> MKKIIYIATIGITLLTTSCDDFLDRQVPQGIVTGDQIASPEYVDNLVISAYAIWATGDDINSSFSLWNYDVRSDDCYKGGSGTEDGGVFNALEISKGINTTDWNINDIWKRLYQCITRANTALQSLDQMDEKTYPLKNQRIAEM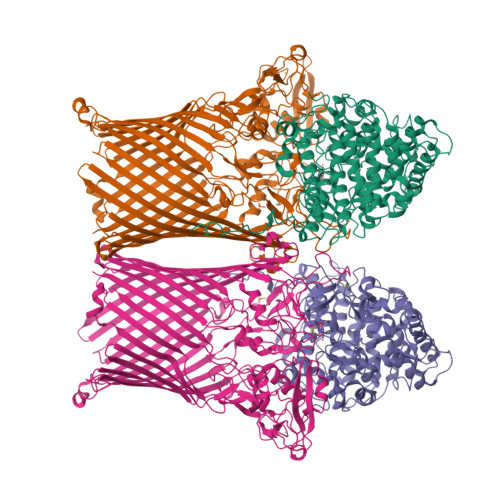RFLRGHAHFMLKQLFKKIVIVNDENMEPDAYNELSNTTYTNDEQWQKIADDFQFAYDNLPEVQIEKGRPAQAAAAAYLAKTYLYKAYRQDGADNALTGINEEDLKQVVKYTDPLIMAKGGYGLETDYSMNFLPQYENGAESVWAIQYSINDGTYNGNLNWGMGLTTPQILGCCDFHKPSQNLVNAFKTDSQGKPLFSTYDNENYEVATDNVDPRLFHTVGMPGFPYKYNEGYIIQKNDDWSRSKGLYGYYVSLKENVDPDCDCLKKGSYWASSLNHIVIRYADVLLMRAEALIQLNDGRITDAISLINEVRSRAAGSTMLIFNYKEDYGVNFKVTPYDLKAYAQDEAMKMLKWERRVEFGMESSRFFDLVRWGEAKDVINAYYVTEASRCSIYKNAGFTENKNEYLPVPFEQISASNGNYTQNFGWAAAAHHHHHH;> MPGIMKNKKLLCSVCFLFAFMSALWGQNITVKGNVTSKTDGQPIIGASVVETTATTNGTITDFDGNFTLSVPVNSTLKITYIGYKPVTVKAAAIVNVLLEEDTQMVDEVVVTGYTTQRKADLTGAVSVVKVDEIQKQGENNPVKALQGRVPGMNITADGNPSGSATVRIRGIGTLNNNDPLYIIDGVPTKAGMHELNGNDIESIQVLKDAASASIYGSRAANGVIIITTKQGKKGQIKINFDASVSASMYQSKMNVLNTEQYGRAMWQAYVNDGENPNGNALGYAYNWGYNADGNPVLYGMTLSKYLDSKNTMPVADTDWFDEITRTGVIQQYNLSVSNGSEKGSSFFSLGYYKNLGVIKDTDFDRFSARMNSDYKLIDDILTIGQHFTLNRTSEVQAPGGIIETALDIPSAIPVYASDGSWGGPVGGWPDRRNPRAVLEYNKDNRYTYWRMFGDAYVNLTPFKGFNLRSTFGLDYANKQARYFTYPYQEGTQTNNGKSAVEAKQEHWTKWMWNAIATYQLEVGKHRGDVMIGMELNREDDSHFSGYKEDFSILTPDYMWPDAGSGTAQAYGAGEGYSLVSFFGKMNYSYADRYLLSLTLRRDGSSRFGKNHRYATFPSVSLGWRITQENFMKELTWLDDLKLRASWGQTGNQEISNLARYTIYAPNYGTTDSFGGQSYGTAYDITGSNGGGVLPSGFKRNQIGNDNIKWETTTQTNVGIDFSLFKQSLYGSLEYYYKKATDILTEMAGVGVLGEGGSRWINSGAMKNQGFEFNLGYRNKTAFGLTYDLNGNISTYRNEILELPETVAANGKFGGNGVKSVVGHTYGAQVGYIADGIFKSQDEVDNHATQEGAAVGRIRYRDIDHNGVIDERDQNWIYDPTPSFSYGLNIYLEYKNFDLTMFWQGVQGVDIISDVKKKSDFWSASNVGFLNKGTRLLNAWSPTNPNSDIPALTRSDTNNEQRVSTYFVENGSFLKLRNIQLGYTVPAVISKKMRMDRLRFYCSAQNLLTIKSKNFTGEDPENPNFSYPIPVNITFGLNIGF> MSITTPEEMIEKAKGETAYLPCKFTLSPEDQGPLDIEW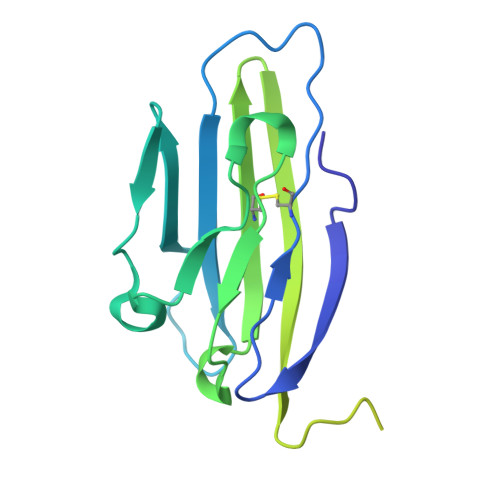LISPADNQKVDQVIILYSGDKIYDDYYPDLKGRVHFTSNDLKSGDASINVTNLQLSDIGTYQCKVKKAPGVANKKIHLVVLVKPSGARCYVDGSEEIGSDFKIKCEPKEGSLPLQYEWQKLSDSQKMPTSWLAEMTSSVISVKNASSEYSGTYSCTVRNRVGSDQCLLRLNVVPPSNKALE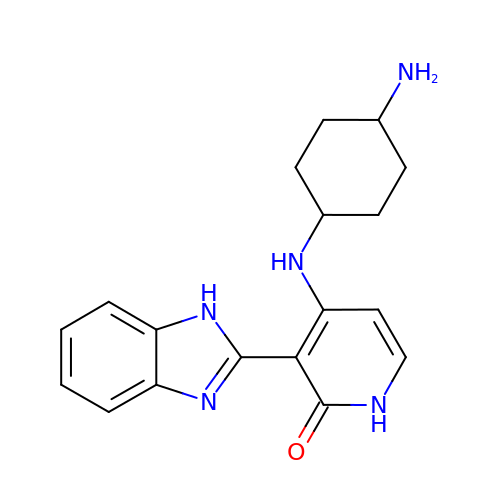4-[(4-aminocyclohexyl)amino]-3-(1H-benzimidazol-2-yl)-1H-pyridin-2-one | C18 H21 N5 O | JLWGOAGEDWMEBT-TXEJJXNPSA-N3-({3-[(6-amino-5-bromopyrimidin-4-yl)sulfanyl]propanoyl}amino)-4-methoxy-N-phenylbenzamide 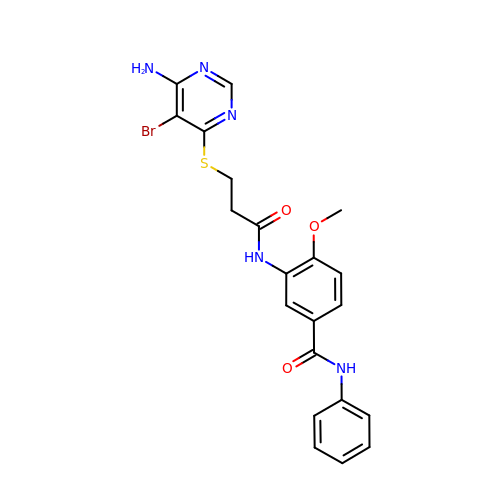| C21 H20 Br N5 O3 S | SSEJHILVXYLIBN-UHFFFAOYSA-N Methionyl-tRNA synthetase (MetRS) is a member of subclass Ia. MetRS is unique among the essential AARSs because it not only charges methionine to tRNA for elongation of translation, but also charges initiator tRNA to initialize translation. MetRS is considered to be one of the most promising drug targets in combatting bacterial pathogens, including MTB. The catalytic domain of MtMetRS spanning residues 1–115 (the N-terminal segment) and residues 226–292 (the C-terminal segment) has a typical α/β Rossmann fold.

We pre-incubated methionine, ATP and Mg2+ with the MtMetRS protein prior to crystallization trials, which allowed the synthesis of an intermediate product in the first step of tRNA charging: methionyl-adenylate (Met-AMP). As expected, we captured a catalytic component complex with Met-AMP fully occupying the active site, providing atomic insight into the recognition of Met-AMP by MtMetRS. The crystals of the MtMetRS–Met-AMP complex diffracted X-rays to 2.4 Å resolution and belonged to space group R3, with a single copy of the enzyme in the asymmetric unit. Our structure reveals that the active site is located on top of the α1 helix and the C-terminal end of the β-strand plane, and is surrounded by helices α2, α3, α7 and α9. The active site can be divided into a binding pocket for methionine and a binding pocket for AMP. While methionine and the ribose and adenosine base parts of Met-AMP are deeply buried, the α-phosphate connecting the adenosine and methionine moieties is more exposed to solvent. The aromatic side chain of Phe292 stabilizes the adenosine base via π–π stacking. In sharp contrast, we found that F-state MtMetRS is characterized by a completely collapsed methionine pocket, a nonexistent AP and a severely reduced groove for adenosine. The binding of Met-AMP induced a conformational change in the nucleotide-binding loop and the active site of MtMetRS was restored to a normal P-state conformation that has no significant differences from the P-state conformation observed in other MetRS homologues. The structure of the MtMetRS–Met-AMP complex demonstrates that the ligand and the CP domain can stabilize the catalytic core and effectively restore the active conformation of the catalytic domain. In the P-state structure, the α2 helix (which is disordered in the apo structure) has a much higher B factor (64.8 Å2) than the average B factor of the entire chain (41.1 Å2), which is unusual for a secondary-structural element.

> MGHHHHHHMKPYYVTTAIAYPNAAPHVGHAYEYIATDAIARFKRLDRYDVRFLTGTDEHGLKVAQAAAAAGVPTAALARRNSDVFQRMQEALNISFDRFIRTTDADHHEASKELWRRMSAAGDIYLDNYSGWYSVRDERFFVESETQLVDGTRLTVETGTPVTWTEEQTYFFRLSAYTDKLLAHYHANPDFIAPETRRNEVISFVSGGLDDLSISRTSFDWGVQVPEHPDHVMYVWVDALTNYLTGAGFPDTDSELFRRYWPADLHMIGKDIIRFHAVYWPAFLMSAGIELPRRIFAHGFLHNRGEKMSKSVGNIVDPVALAEALGVDQVRYFLLREVPFGQDGSYSDEAIVTRINTDLANELGNLAQRSLSMVAKNLDGRVPNPGEFADADAALLATADGLLERVRGHFDAQAMHLALEAIWLMLGDANKYFSVQQPWVLRKSESEADQARFRTTLYVTCEVVRIAALLIQPVMPESAGKILDLLGQAPNQRSFAAVGVRLTPGTALPPPTGVFPRYQPPQPPEGKRS> PLNKFPGFAKPGTEQYLLAKQLAKPKEKIPIIVGDYGPMWVYPTSTFDCVVADPRKGSKMYGLKSYIEYQLTPTNTNRSVNHRYKHFDWLYERLLVKFGSAIPIPSLPDKQVTGRFEEEFIKMRMERLQAWMTRMCRHPVISESEVFQQFLNFRDEKEWKTGKRKAERDELAGVMIFSTMEPEAPDLDLVEIEQKCEAVGKFTKAMDDGVKELLTVGQEHWKRCTGPLPKEYQKIGKA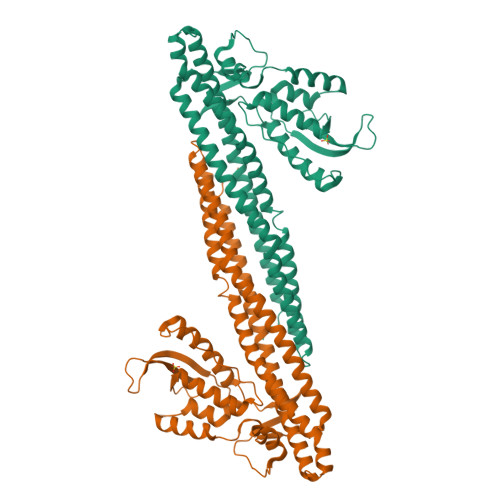LQSLATVFSSSGYQGETDLNDAITEAGKTYEEIASLVAEQPKKDLHFLMECNHEYKGFLGCFPDIIGTHKGAIEKVKESDKLVATSKITLQDKQNMVKRVSIMSYALQAEMNHFHSNRIYDYNSVIRLYLEQQVQFYETIAEKLRQALSRFPVM> TTPLVHVASVEKGRSYEDFQKVYNAIALKIAEKKCGPVLV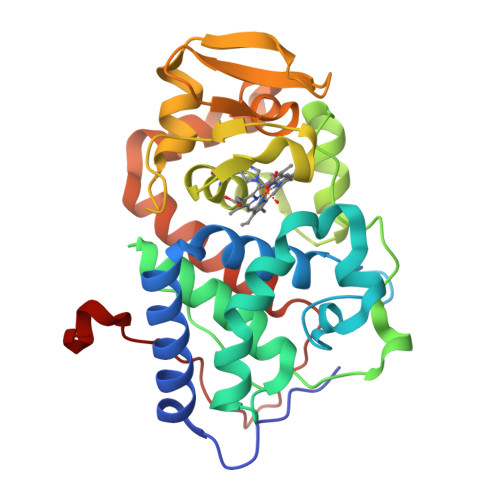RLAWHTSGTWDKHDNTGGSYGGTYRFKKEFNDPSNAGLQNGFKFLEPIHKEFPWISSGDLFSLGGVTAVQEMQGPKIPWRCGRVDTPEDTTPDNGRLPDADKDADYVRTFFQRLNMNDREVVALMGAHALGKTHLKRSGYEGPFGAANNVFTNEFYLNLLNEDWKLEKNDANNEQWDSKSGYMMLPTDYSLIQDPKYLSIVKEYANDQDKFFKDFSKAFEKLLENGITFPKDAPSPFIFKTLEEQGL> VVGGEDAK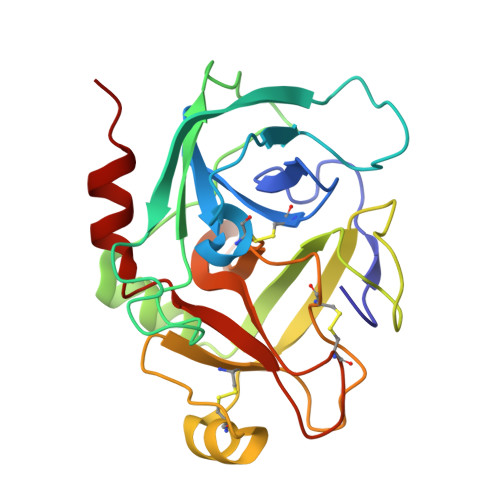PGQFPWQVVLNGKVDAFCGGSIVNEKWIVTAAHCVETGVKITVVAGEHNIEETEHTEQKRNVIRIIPHHNFNAAINTYNHDIALLELDEPLVLNSYVTPICIADKEYTNIFLKFGSGYVSGWGRVFHKGRAALVLQYLRVPLVDRATCLRSTKFTITNNMFCAGFHEGGRDSCQGDSGGPHVTEVEGTSFLTGIISWGEECAMKGKYGIYTKVSRYVNWIKEKTKLT>[28x]MKYVVVSGGVISGIGKGVLASSTGMLMKTLGLKVTSIKIDPYMNIDAGTMSPLEHGECFVLDDGGETDLDLGNYERYLGVTLTKDHNITTGKIYSHVIAKERKGDYLGKTVQIVPHLTNAIQDWIERVAKIPVDDTGMEPDVCIIELGGTVGDIESAPFVEALRQFQFKVGKENFALIHVSLVPVIHGEQKTKPTQAAIKGLRSLGLVPDMIACRCSETLDKPTIDKIAMFCHVGPEQVVNVHDVNSTYHVPLLLLEQKMIDYLHARLKLDEITEEEKQRGLELLSKWKATTGNFDEETVKIALVGKYTNLKDSYLSVIKALEHSSMKCRRKLDIKWVEATDLEPEAQESNKTKFHEAWNMVSTADGILIPGGFGVRGTEGMVLAARWARENHIPFLGVCLGLQIATIEFTRSVLGRKDSHSAEFYPDIDEKNHVVVFMMRLGLRPTFFQNETEWSQIKKLYGDVSEVHERHRHRYEINP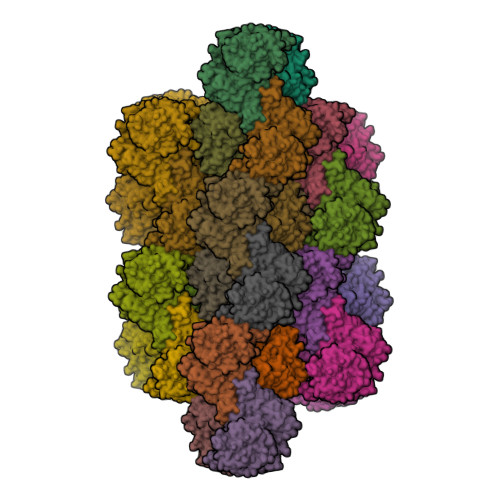KMVDELENNGLIFVGKDDTGKRCEILELKNHPYYIATQYHPEYTSKVLDPSKPFLGLVAASAGILQDVIEGKYDLEA> SGSGKPAYQIYMEFFQNKQDDHDPIDTFVIQKRALLAQLPSGRHDEETELDLLFGLLNIKYRKHISRHSVHTFKDLLEQGRIIEHNNQED

One of the key proteins in long-term synaptic plasticity and memory is the activity-regulated cytoskeleton-associated protein (Arc). Drosophila has two isoforms of Arc, dArc1 and dArc2, with low sequence similarity to mammalian Arc, but lacking a large N-terminal domain. Both dArc isoforms are related to the Ty3/gypsy retrotransposon capsid, consisting of N- and C-terminal lobes. As opposed to the corresponding mammalian Arc lobe domains, which are monomeric, the dArc lobes were all oligomeric in solution, indicating a strong propensity for homophilic interactions.

Each monomer consists of five helices in an orthogonal bundle fold, and the structures are highly similar to each other. The dimer interface is in both cases formed by α1 and α3 from each monomer, and the total buried surface area at the interface is ~1400 Å2. Both interfaces contain four hydrogen bonds and four salt bridges. The interface is conserved, displaying only three conservative replacements between the isoforms (A125/L170/F172 in dArc1 to S112/F157/Y159 in dArc2). (D) A comparison of the dArc-CL crystal structures with the same domains in dArc capsids. Both the dArc1 and dArc2 C-lobes closely resemble their counterparts in the capsids, with an all-atom RMSD of 1.75 Å2 and 1.13 Å2, respectively. The dimer interface in dArc-CL, which corresponds to that in retroviral CA-CTD, contains mainly hydrophobic interactions; half of these hydrophobic residues are polar in the rat Arc-CL, and the first helix of the dArc-CL, a major part of the dimer interface, is tilted away in mArc, possibly explaining the monomeric state of mArc-CL in solution. CD spectra of the dArc C-lobes are similar but differ in intensity, suggesting that dArc1-CL is less folded in solution, despite the very similar crystal structures. Kratky plots also indicate that dArc1-CL is more flexible than dArc2-CL.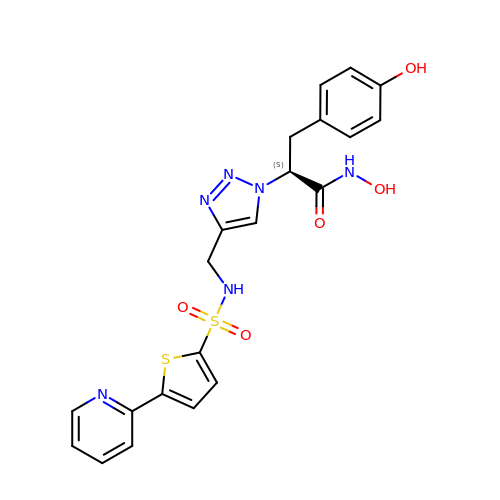(2~{S})-3-(4-hydroxyphenyl)-~{N}-oxidanyl-2-[4-[[(5-pyridin-2-ylthiophen-2-yl)sulfonylamino]methyl]-1,2,3-triazol-1-yl]propanamide | C21 H20 N6 O5 S2 | QHHWCHMBFWYFFS-SFHVURJKSA-N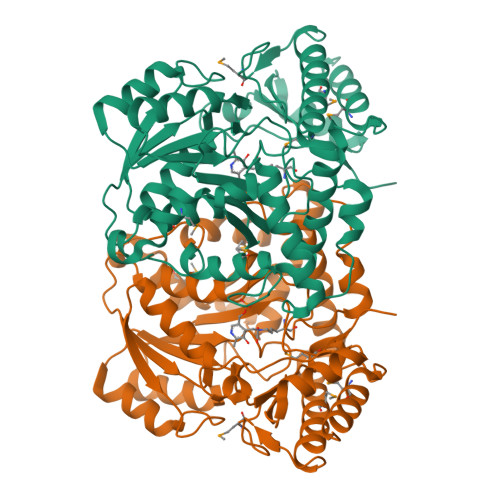> MTKSVDTLLIPGPIILSGAVQKALDVPSLGHTSPEFVSIFQRVLKNTRAVFKSAAASKSQPFVLAGSGTLGWDIFASNFILSKAPNKNVLVVSTGTFSDRFADCLRSYGAQVDVVRPLKIGESVPLELITEKLSQNSYGAVTVTHVDTSTAVLSDLKAISQAIKQTSPETFFVVDAVCSIGCEEFEFDEWGVDFALTASQKAIGAPAGLSISLCSSRFMDYALNDSKNGHVHGYFSSLRRWTPIMENYEAGKGAYFATPPVQLINSLDVALKEILEEGLHKRWDLHREMSDWFKDSLVNGLQLTSVSRYPSNMSAHGLTAVYVADPPDVIAFLKSHGVVIAGGIHKDIGPKYIRIGHMGVTACNKNLPYMKNCFDLIKLALQRKK>ADTIVAVELDTYPNTDIGDPSYPHIGIDIKSVRSKKTAKWNMQNGKVGTAHIIYNSVGKRLSAVVSYPNGDSATVSYDVDLDNVLPEWVRVGLSASTGLYKETNTILSWSFTSKLKSNSTHETNALHFVFNQFSKDQKDLILQGDATTGTDGNLELTRVSSNGSPQGSSVGRALFYAPVHIWESSAVVASFDATFTFLIKSSDSHPADGIAFFISNIDSSIPSG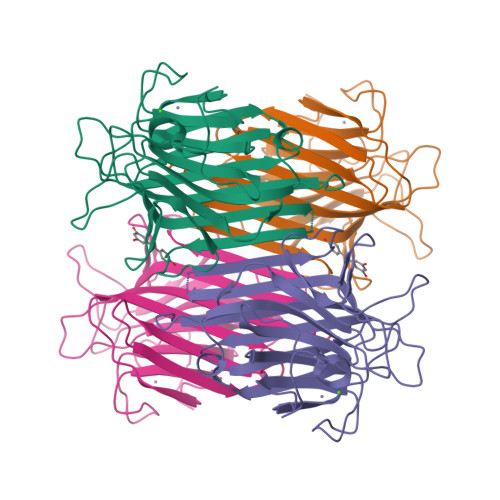STGRLLGLFPDAN[2x]BET proteins are chromatin-associated factors that regulate transcription and chromatin remodelling. BET proteins bind chromatin through their two BDs (BD1 and BD2), which specifically recognize histones acetylated on lysine residues. The BDs from C. albicans Bdf1 (CaBdf1) share 31–46% sequence identity with human BET BDs and 58–66% identity with those from ScBdf1 and hence are likely to bind multi-acetylated H3 and H4 tails. In conclusion, Bdf1 BDs are required for the viability and virulence of C. albicans and can be selectively targeted by small-molecule inhibitors without compromising human BET BD function.

In particular, several compounds possessing a dibenzothiazepinone scaffold exhibited low-micromolar IC50 values towards CaBdf1 BD1 and no or only weak inhibition of Brd4 BD1 at the highest concentration (20 μM) tested. One such inhibitor was compound 1. ITC measurements showed that 1 binds CaBdf1 BD1 with a Kd of 5 μM, consistent with the IC50 value (4.3 μM) determined by HTRF, whereas no or only modest binding and inhibition were detected for Brd4 BD1 and CaBdf1 BD2. Furthermore, a BROMOscan screen from DiscoverX revealed that compound 1 showed no significant activity against 32 representative human (BET and non-BET) BDs; indeed, an ITC experiment confirmed that the two human BDs (SMARCA2 and SMARCA4) with the strongest BROMOscan response did not detectably bind compound 1. To understand the molecular basis of selectivity we solved the crystal structure of CaBdf1 BD1 bound to 1. Compound 1 mimics the acetyllysine ligand by interacting with the conserved Tyr248 and Asn291 residues, forming direct and water-mediated hydrogen bonds via the thiazepinone carbonyl group. The dibenzothiazepinone ring system engages hydrophobic residues from the Val-Pro-Phe (VPF) shelf (Pro233), helix B (Phe290) and the ZZ′ loop (Val238, Leu243 and Val245), while the cyclopropyl group interacts with the VPF shelf (Pro233 and Phe234), helix B (Cys287) and the gatekeeper residue on helix C (Ile297). In contrast, the oxadiazole and pyrazine groups point away from the pocket, adopting different orientations in the four complexes present in the crystal's asymmetric unit. Superimposing the ligand-bound structure with that of Brd4 BD1 results in a steric overlap between the larger Brd4 side chains at signature positions 1 and 3 (Trp81 and Leu94) and the oxadiazole and distal benzene groups of compound 1, explaining why 1 fails to inhibit the human BD. Steric hindrance from the corresponding residues in CaBdf1 BD2 (Phe409 and Ile422) also account for this domain's insensitivity to compound 1.

>AAGAPKPPQEPDMNNLPENPIPQHQAKFVLNTIKAVKRNREAVPFLHPVDTVKLNVPFYYNYIPRPMDLSTIERKINLKAYEDVSQVVDDFNLMVKNCKKFNGEAAGISKMATNIQAQFEKLMVKVPPKELPAGTNVA[4x]> MHHHHHHGENLYFQGSWESKFAKESLTFDDVLLIPAQSDILPKDVDLSVQLSDKVKLNIPVISAGMDTVTESKMAIAMARQGGLGVIHKNMGVEEQADEVQKVKRSGGLLVAAAIGISKDTDIRAQKLVEAGVDVLVIDTAHGHSKGVIDQVKHIKKTYPEITLVAGNVATAEATKDLFEAGADIV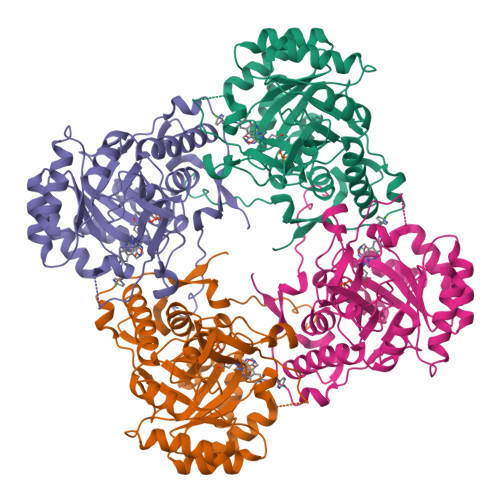KVGIGPGSICTTRVVAGVGVPQITAIYDCATEARKHGKAIIADGGIKFSGDIIKALAAGGHAVMLGSLLAGTEESPGATEIFQGRQYKVYRGMGSLGAMEKGSNDRYFQEDKAPKKFVPEGIEGRTAYKGALQDTIYQLMGGVRAGMGYTGSHDLRELREEAQFTRMGPAGLAESHPHNIQITKESPNYSFGNS>[8x]MKIAVLSRNPRLY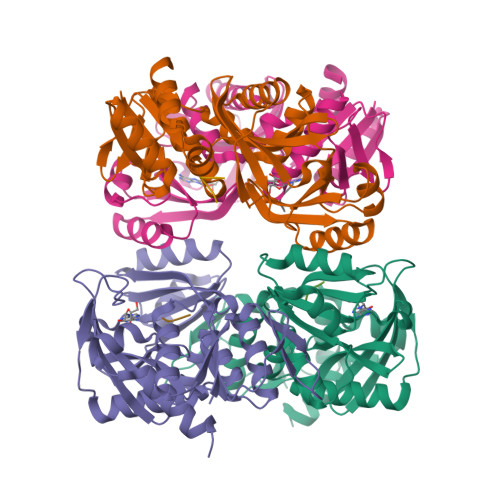STRRLVEAGRERGHEMVVIDTLRAYMNIASHKPQIHYRGQPLEGFDAVIPRIGASVTFYGCAVLRQFEMMGVFPLNESVAIARSRDKLRSLQLLSRKGIGLPVTGFAHSPDDVPDLIEMVGGAPLVIKLLEGTQGIGVVLCETEKAAESVLEAFMGLKHNIMVQEYIKEAGGADIRCFVVGDKVIASMKRQAAPGEFRSNLHRGGSASLIKITPEERMTAIRAARVMGLNVAGVDILRSNHGPLVMEVNSSPGLEGIESTTGKDIAGIIIQYLEKNGGPHLARTKGKGKLAAALEHHHHHH;>[8x]EEEEEEEEEEEEEEEEEEEEEEEEEEEEEEEEEEEEEEEEEEEEEEEEEEEEEEEEEEEE> MHHHHHHHHMVTVAVPKERAPGERRVALVPEVVARLVKGGARVR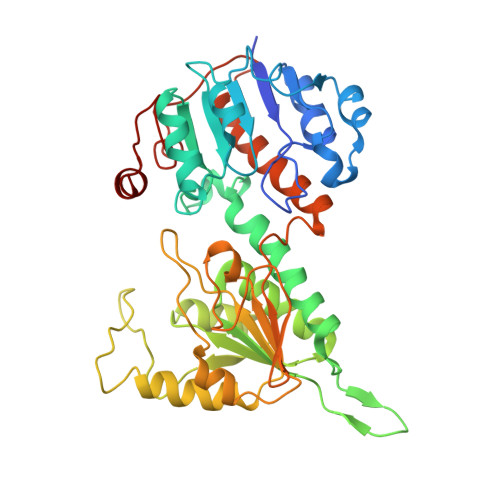VERGAGEGAYHPDEAYQEAGAEVVERGELLKGAHLLFTVQPPPEDLIQALEPGAIVVGFVQPHKNLELVRALQAKKATVIAMELIPRITRAQSMDALSSQATVAGYLAAIHAARLSPRFFPMLTTAAGTIRPAKVMVMGVGVAGLMAIATAKRLGAQVFAYDVRKAALEQALSLGAKPIELPISAEGEGGYARELTEEEKRIQHEALRDHVAGMDVLITTAQVPGRRAPILLTEDMVERLKPGTVVVDLAAESGGNCVLTKPGEVVEVRGVRVYGPLNLPSELSVHASEMYAKNLYNLSSLLIEKGAFAPKWEDEIVRAALLMKEGEVLHGPTKALLGGA> GGSEVRILLLGLDNAGKTTLLKQLASEDISHITPTQGFNIKSVQSQGFKLNVWDIGGLRKIRPYWRSYFENTDILIYVIDSADRKRFEETGQELTELLEEEKLSCVPVLIFANKQDLLTAAPASEIAEGLNLHTIRDRVWQIQSCSALTGEGVQDGMNWVCKNV;> GSMGCFFSKRRKADKESRPENEEERPKQYSWDQREKVDPKDYMF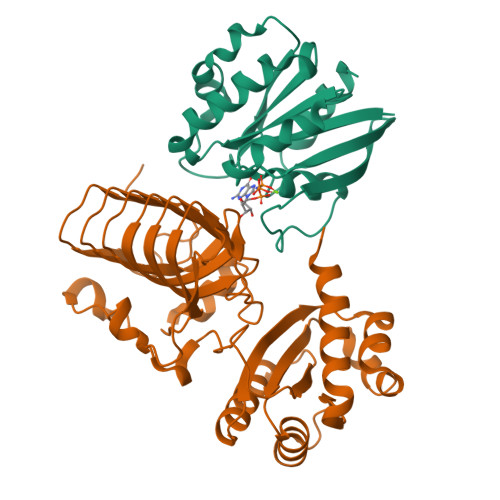SGLKDETVGRLPGTVAGQQFLIQDCENCNIYIFDHSATVTIDDCTNCIIFLGPVKGSVFFRNCRDCKCTLACQQFRVRDCRKLEVFLCCATQPIIESSSNIKFGCFQWYYPELAFQFKDAGLSIFNNTWSNIHDFTPVSGELNWSLLPEDAVVQDYVPIPTTEELKAVRVSTEANRSIVPISRGQRQKSSDESCLVVLFAGDYTIANARKLIDEMVGKGFFLVQTKEVSMKAEDAQRVFREKAPDFLPLLNKGPVIALEFNGDGAVEVCQLIVNEIFNGTKMFVSESKETASGDVDSFYNFADIQMGI~{N}-[(3~{S})-2,5-bis(oxidanylidene)pyrrolidin-3-yl]-3-phenyl-propanamide | C13 H14 N2 O3 | 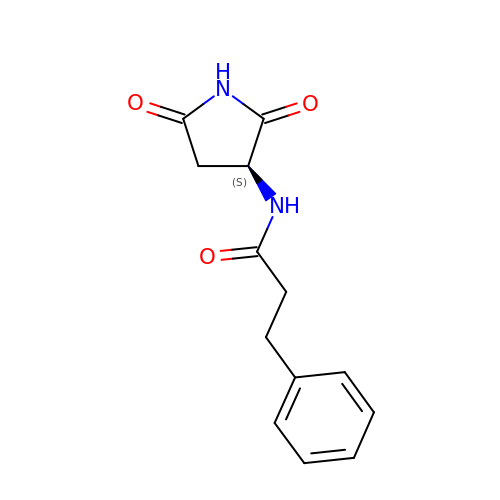VPQQSXIHDPBURE-JTQLQIEISA-N> MGSDSIDTPNYDVQKHINKLCGMLLITEDANHKFTGLIGMLYAMSRLGREDTIKILRDAGY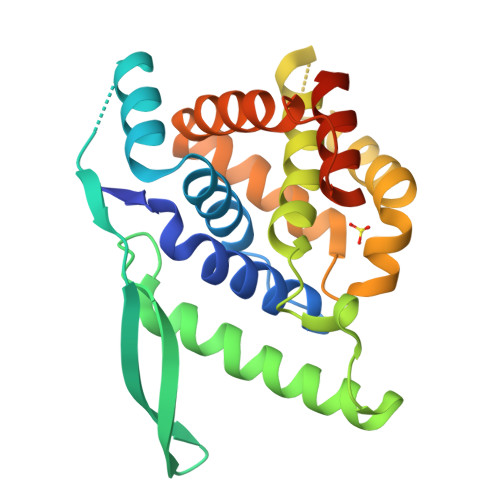HVKANGVDVTTHRQDINGKEMKFEVLTLASLTTEIQINIEIESRKSYKKMLKEMGEVAPEYRHDSPDCGMIILCILALVITKLAAGDRSGLTAVIRRANNVLKNEMKRYKGLLPKDIANSFYEVFEKHPHFIDVFVHFGIAQSSTRGGSRVEGIFAGLFMNAYGLEHHHHHH;> MGSDSIDTPNYDVQKHINKLCGMLLITEDANHKFTGLIGMLYAMSRLGREDTIKILRDAGYHVKANGVDVTTHRQDINGKEMKFEVLTLASLTTEIQINIEIESRKSYKKMLKEMGEVAPEYRHDSPDCGMIILCIAALVITKLAAGDRSGLTAVIRRANNVLKNEMKRYKGLLPKDIANSFYEVFEKHPHFIDVFVHFGIAQSSTRGGSRVEGIFAGLFMNAYGLEHHHHHH>GPLGSSEDYRDTVVKRKPASLMAPLKRKEEFSLFKVSDDEYKVTIS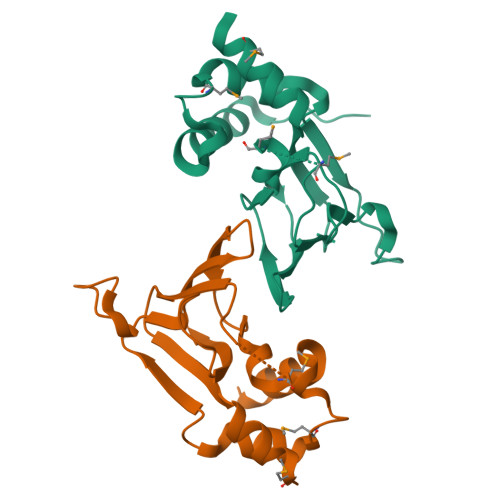PQLLLATQRFLSREVDVFSPLRMSEKVLLHLLKHPSVNQEVRFDESNRLATHHYLYQRSQPVDYFILILQGRVEVEIGKEGLKFENGAFTYYGVSALMVPSSVHQSPVSSLQPIRHDLQPDPGDGTHSSMYCPDYTVRALSDLQLIKVTRLQYLNALMATRAQNLPQSPENTDLQMMPGSQTRLLGEKTTTAAGSSHSRPGVPVEGSPGRNPGV[2x]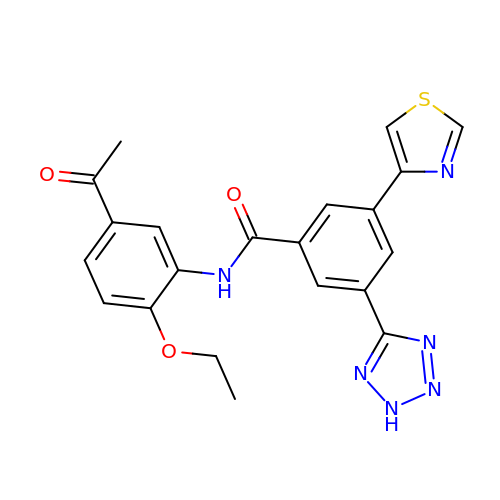~{N}-(5-ethanoyl-2-ethoxy-phenyl)-3-(2~{H}-1,2,3,4-tetrazol-5-yl)-5-(1,3-thiazol-4-yl)benzamide | C21 H18 N6 O3 S | BCRZPXIIINLQPD-UHFFFAOYSA-N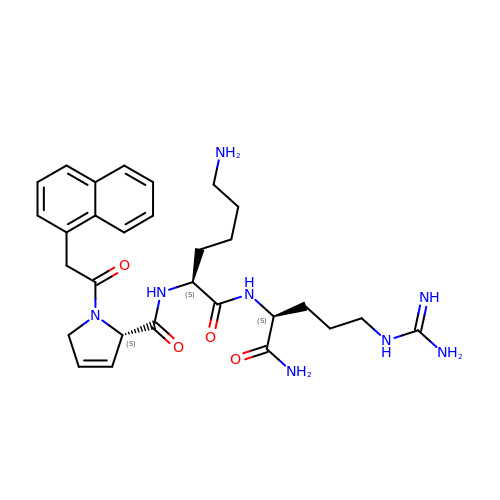N~2~-{(2S)-1-[(naphthalen-1-yl)acetyl]-2,5-dihydro-1H-pyrrole-2-carbonyl}-L-lysyl-L-argininamide | C29 H40 N8 O4 | FRFITSHXIRHPKA-HJOGWXRNSA-N>[3x]MTTATAGLAVELKQSTAQAHEKAEHSTFMSDLLKGRLGVAEFTRLQEQAWLFYTALEQAVDA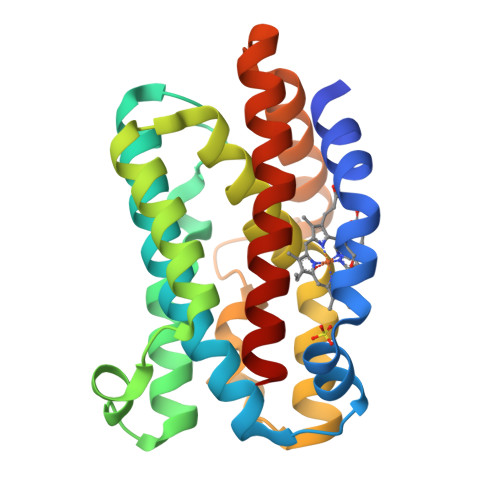VRASGFAESLLDPALNRAEVLARDLDKLNGSSEWRSRITASPAVIDYVNRLEEIRDNVDGPALVAHHYVRYLGALSGGQVIARMMQRHYGVDPEALGFYHFEGIAKLKVYKDEYREKLNNLELSDEQREHLLKEATDAFVFNHQVFADLGKGL>[2x]MKKLQIAVGIIRNENNEIFITRRAADAHMANKLEFPGGKIEMGETPEQAVVRELQEEVGITPQHF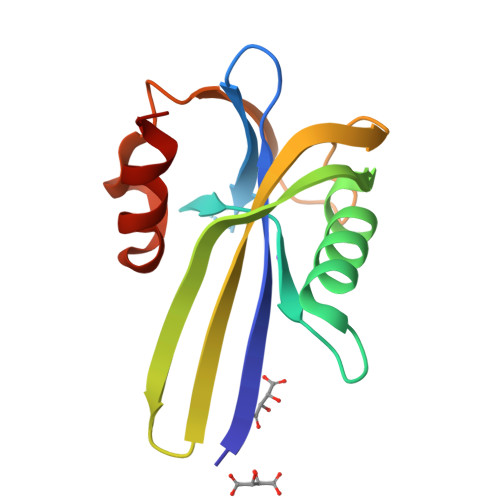SLFEKLEYEFPDRHITLWFWLVERWEGEPWGKEGQPGEWMSLVGLNADDFPPANEPVIAKLKRL> MHHHHHHNEIVVKGARVHNLKNITVRIPKNRLVVITGVSGSGKSSLAMDTIYAEGQRRYLESLSTYARQFLGNLKKPDVDEIEGLSPAIAIDQKTVSHNPRSTVGTVTEIYDYLRVLYARIGKKINGLNIHEFTELSISEELEFLKNLNLTEREREIVGELLKEIEKRLEFLVDVGLEYLTLSRSATTLSGGESQRIRLATQIGSGLTGVIYVLDEPTIGLHPRDTERLIKTLKKLRDLGNTVIVVEHDEEVIRNADHIIDIGPGGGTNGGRVVFQGTVDELLKNPDSSLTGEYLSGKRKITVNKTRRLPYASLKIKGVRHNNLKNIDVEIPLGVFVCVTGVSGSGKSSLVMETLYPALMNLLHKTKLPAGEFDSIEGHENIDKMIAIDQSPIGRTPRSNPATYTKVFDEIRSLFAMTPAAKARGYNKSRFSFNLKGGRCEACQGQGYVKIEMLFLPDVYVECDVCKGKRYNRETLEITYKGKNISDILDMTVDEALEFFKNIPSIKRTLQVLHDVGLGYVKLGQPATTLSGGEAQRIKLASELRKRDTGRTLYILDEPTVGLHFEDVRKLVEVLHRLVDRGNTVIVIEHNLDVIKNADHIIDLGPEGGKEGGYIVATGTPEEIAKNPHSYTGRFLKNVL

The UvrA2 dimer finds lesions in DNA and initiates nucleotide excision repair. UvrA2 is also an ATPase from the ATP-binding cassette (ABC) family of proteins, which have a distinctive composite nucleotide-binding site for coupling ATP binding and hydrolysis to conformational changes. UvrA2 is an unusual member of this family in that it has two ATPase sites per monomer instead of one, resulting in a total of four sites on the dimer. The two sites on each monomer are termed ‘proximal’ and ‘distal’, and each site comprises an ATP-binding domain with Walker A and B motifs and a signature domain with the ABC signature motif.

UvrA2 structures from different organisms have been determined in nucleotide-free, P2ADP-D2ADP or Pempty-D2ADP state, with most in open conformation (including the T. maritima UvrA2 structure reported here) with a shallow and wide DNA binding surface, and one structure (in complex with UvrB) in closed conformation with a deep and narrow DNA binding surface. UvrA2 structures determined in open form are in either nucleotide-free, fully ADP-bound or, in one case, in Pempty-D2ADP state, suggesting that ATP hydrolysis by one or both ATPase sites favors this conformation (the fully ADP-bound structure reported here further supports this hypothesis). Nucleotide-bound/free UvrA2 structures reveal signature domain II in different conformations, suggesting it could affect ATPase-driven changes in UvrA2 interactions with DNA and UvrB. Such dynamism has not been reported for distal site signature domain I. A C-terminal zinc-binding hairpin within the proximal site signature domain II also adopts different conformations and is implicated in ATPase-modulated interactions of UvrA2 with damaged DNA (the UvrA2 structure reported here shows the hairpin in a new, intermediate position). To gain additional insights into the finding that nucleotides are held more tightly by the distal ATPase sites than proximal sites, we interrogated atomic models of several UvrA2 orthologs for underlying sources of the differential affinity. Detailed examination of the complete set of contacts between UvrA2 and nucleotide at all the sites revealed 21 polar and 28 hydrophobic contacts per site, on average (both proximal and distal sites make 21 polar contacts, and 29 and 27 hydrophobic contacts, respectively). These contacts are highly conserved between the two types of sites and between orthologs, with one notable exception. The proximal site has a glutamine residue that precedes the ABC signature motif by five residues (Q821, G. stearothermophilus residue numbering). In contrast, the distal ATPase site of every UvrA2 ortholog features an arginine in the equivalent position, which is involved in a pi–cation interaction with the aromatic base of adenine (R480). While both residues stack on the adenine base, the more extensive interaction and pi–cation stacking by R480 implicate this residue in the higher affinity of distal sites for nucleotides.>GHAPDKIVLDHAFGQTILDKKPERVATIAWGNHDVALALGIVPVGFSKANYGVSADKGVLPWTEEKIKELNGKANLFDDLDGLNFEAISNSKPDVILAGYSGITKEDYDTLSKIAPVAAYKSKPWQTLWRDMIKIDSKALGMEK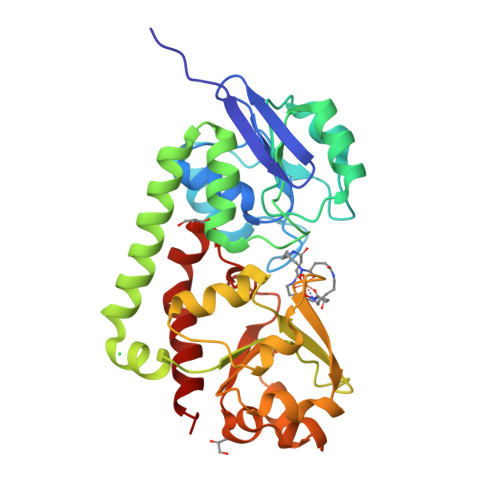EGDELIKNTEARISKELEKHPEIKGKIKGKKVLFTMINAADTSKFWIYTSKDPRANYLTDLGLVFPESLKEFESEDSFAKEISAEEANKINDADVIITYGDDKTLEALQKDPLLGKINAIKNGAVAVIPDNTPLAASCTPTPLSINYTIEEYLNLLGNACKNAK[2x]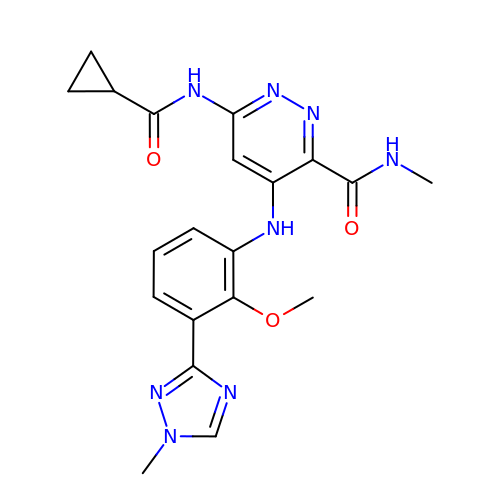6-[(cyclopropanecarbonyl)amino]-4-{[2-methoxy-3-(1-methyl-1H-1,2,4-triazol-3-yl)phenyl]amino}-N-methylpyridazine-3-carboxamide | C20 H22 N8 O3 | BZZKEPGENYLQSC-UHFFFAOYSA-N>GFDYDVVVVGGGFAGATAARECGLQGYRTLLLEARSRLGGRTFTSRFAGQEIELGGTWVHWLQPHVWAEMQRYGLGVVEDPLTNLDKTLIMYNDGIVESISPDEFGKNIRIAFEKLCHDAWEVFPRPHEPMFTERARELDK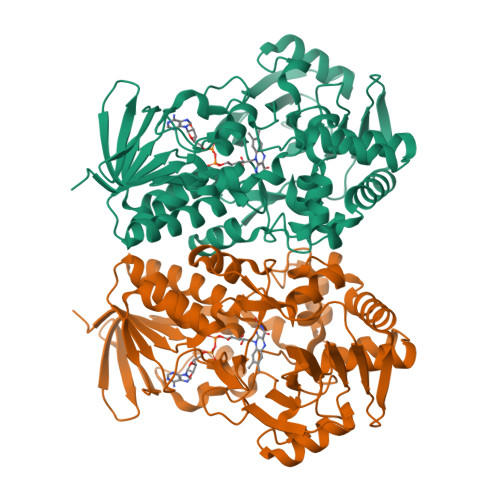SSVLDRIKTLGLSRLQQAQINSYMALYAGETTDKFGLPGVLKLFACGGWNYDAFMDTETHYRIQGGTIGLINAMLTDSGAEVRMSVPVTAVEQVNGGVKIKTDDDEIITAGVVVMTVPLNTYKHIDFTPALSKGKQRFIKEGQLSKGAKLYVHVKQNLGRVFAFADEQQPLNWVQTRDYSDELGTILSITIARKETIDVNDRDAVTREVQKMFPGVEVLGTAAYDWTADPFSLGAWAAYGVGQLSRLKDLQAAEGRIVFAGAETSNGWHASIDGAVESGLRAGREVKQLLS[2x]> RSFSSRTPVNENPDGVQYRRGFVTRHQVSGWRFVMRRIASGVALHDTRMLVDPLRTQSRAVLTGALILVTGLVGCFIFS;>[2x]PIVRVAVLAAGDDGGRLTEMALPSELPLREILPAVQRIVQPARENDGAADPAAAPNPVRLSLAPIGGAPFSLDATLDTVGVVDGDLLALQAVPSGPPAPRIVEDIADAAVIFSEARRRQWGPTHIARGAALALIGLILVGTGLSVAHRVITGDLLGQFIVSGIALATVIAALAVRNR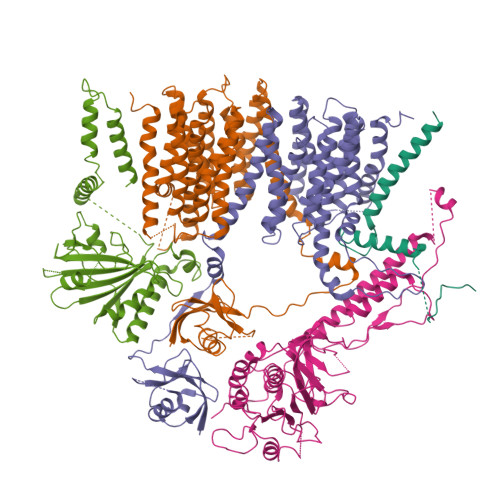SAVLATSLAVTALVPVAAAFALGVPGDFGAPNVLLAAAGVAAWSLISMAGSPDDRGIAVFTATAVTGVGVLLVAGAASLWVISSDVIGCALVLLGLIVTVQAAQLSAMWARFPLPVIPAPGDPTPAARPLSVLADLPRRVRVSQAHQTGVIAAGVLLGVAGSVALVSSANASPWAWYIVVAAAAGAALRARVWDSAACKAWLLGHSYLLAVALLVAFVIGDRYQAALWALAALAVLVLVWIVAALNPKIASPDTYSLPMRRMVGFLATGLDASLIPVMALLVGLFSLV;> SRLIFEHQRRLTPPTTRKGTITIEPPPQLPRVVPPSLLRRVLPFLIVILIVGMIVALFATGMRLISPTMLFFPFVLLLAATALYRGGDNKMRTEEVDAERADYLRYLSVVRDNVRAHAAEQRAALEWSHPEPEVLATIPGTRRQWERDPRDRDFLVLRAGRHDVPLDAALKVKDTADEIDLEPVAHSALRGLLDVQRTVRDAPTGLDVAKLARITVIGEADEARAAIRAWIAQAVTWHDPTMLGVALAAPDLESGDWSWLKWLPHVDVPNEADGVGPARYLTTSTAELRERLAPALADRPLFPAESGAALKHLLVVLDDPDADPDDIARKPGLTGVTVIHRTTELPNREQYPDPERPILRVADGRIERWQVGGWQPCVDVADAMSAAEAAHIARRLSRWDS;> MTARIALASLFVVAAVLAQPWQTTTQRWVLGVSIAAVIVLLAWWKGMFLTTRIGRALAMVRRNRAEDTVETDAHRATVVLRVDPAAPAQLPVVVGYLDRYGITCDKVRITHRDAGGTRRSWISLTVDAVDNLAALQARSARIPLQDTTEVVGRRLADHLREQGWTVTVVEGVDTPLPVSGKETWRGVADDAGVVAAYRVKVDDRLDEVLAEIGHLPAEETWTALEFTGSPAEPLLTVCAAVRTSDRPAAKAPLAGLTPARGRHRPALAALNPLSTERLDGTAVPL>GSMRFLYHPDRKDISLPGVLYALGDPARLEIVRLLASKG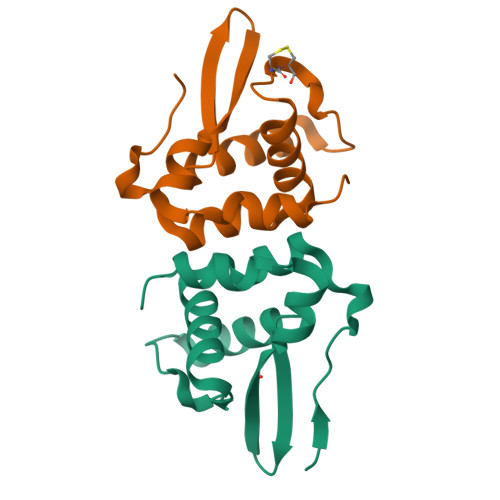EQCCAEFDFAIAKSTMSNHFKILRESGVVLTRKEGTQHINRLRREDLETLFPGLLDAVLRSAQPLLTCQQSAIVK[2x]>[4x]GS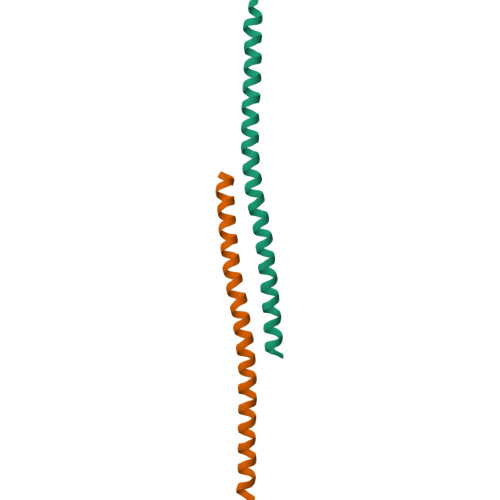ESGDNVRSSAGAVRDAGGAFGKREQAEEERYFRARAKEQLAALKKHKENEISHHAKEIERLQKEIERHKQSIKKLKQSEDDD>[8x]MASRGSHHHHHHGAYRLLNKTAVITGGNSGIGLATAKRFVAEGAYVFIVGRRRKELEQAAAEIGRNVTAVKADVTKLEDLDRLYAIVREQRGSIDVLFANSGAIEQKTLEEITPEHYDRTFDVNVRGLIFTVQKALPLLRDGGSVILTSSVAGVLGLQAHDTYSAAKAAVRSLARTWTTELKGRSIRVNAVSPGAIDTPIIENQVSTQEEADELRAKFAAATPLGRVGRPEELAAAVLFLASDDSSYVAG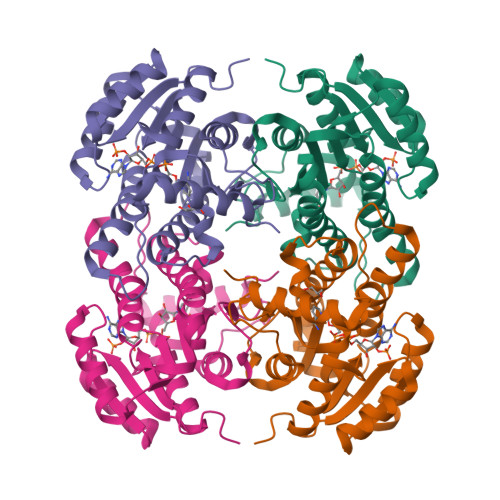IELFVDGGLTQV>[10x]GASKAFYSAGDKLFQPGDDAVASMQTYSVAQFLQPFTLNPAKASSDYLGKWVKVRGVIVDIRRKSGIAGSYYFIVTMRDEQNKTDKRLTFNFGSHN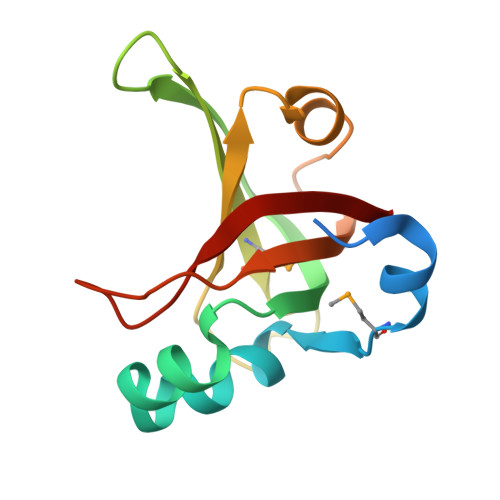SADVEALSNGSVATIVGQVHQVQDSTIPTLQNPKVVK>[2x]GHMGQIPLKEVTFARLNDNVRETFLKDMCRKYGEVEEVEILLHPRTRKHLGLARV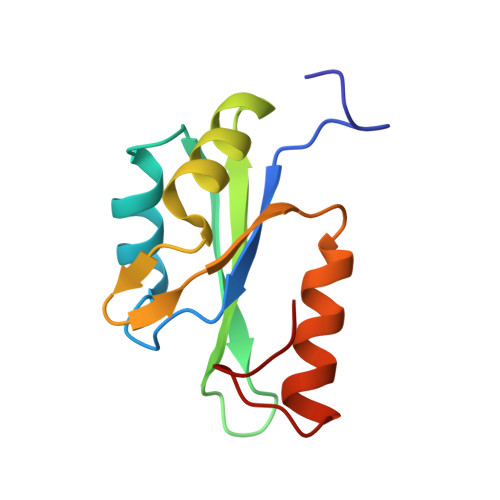LFTSTRGAKETVKNLHLTSVMGNIIHAQLDIKGQQRMKYYELIVNGSYTPQTVPT> GHMSKSDYIQNMFQTKSFVDRYKYTEKLTGLYAQTLVDYSGVANTSQKPLIVLDNACGIGAVSSVLNHTLQDEAKKTWKLTCGDLSEGMLETTKRRLQDEGWVNAETKIVNALDTGLPDGHYTHVFVAFGFQSFPDANAALKECFRILASGGILASSTWQNFNWIPIMKAAIETIPGNLPFPTQKEFIALHNAGWDSESYIQSELEKLGFRDVKVIPVPKETSIPIDEFFEVCMMIIPYLLPKFWTEEQRESHEKDVPMVLRQYLQDTYGANGQVPLEAVALITTGLKP

We and others have shown that A. fumigatus effects dithiol gliotoxin S-methylation via a methyltransferase, gliotoxin thiomethyltransferase A (GtmA or TmtA) located outside the gliotoxin gene cluster. GtmA consists of two domains, a larger ‘upper’ domain containing a Rossmann-fold involved in binding the co-substrate SAM and a smaller ‘lower’ domain that changes its relative position to the upper domain in the three crystal structures described here. apo-GtmA seems to be highly flexible, as indicated by the higher B-factors. In agreement with Duell et al., who have recently published the structure of a GtmA–SAH complex in the same crystal form as described here, the cofactor binding site of GtmA is located in the upper part of a cleft between the two domains built by helix α1, sheet β2 and loop regions connecting β1–α2 and β3–β4. Our data suggest that GtmA methylates dithiol gliotoxin by a non-processive mechanism.

In order to obtain detailed insights into the enzymatic mechanism of GtmA-catalysed methyltransfer, we crystallized GtmA in the cofactor-free form and in complex with SAM and SAH, and refined the structures at 1.66 Å, 2.28 Å and 1.33 Å resolution with R-factors of Rapo = 16.8, RSAM = 19.2, RSAH = 13.9, and Rfree-values of Rfreeapo = 18.6, RfreeSAM = 23.4, RfreeSAM = 16.6, respectively. The apo form crystallized in space group P62 with one chain in the asymmetric unit, whereas the complexes appeared in two different crystal forms belonging to space group P21 with two monomers as the asymmetric unit in both cases. The flexibility is more pronounced in the lower domain, which is also evident by the finding that almost no ordered water molecules can be observed in the electron density of this region. The apo structure adopts a similar conformation as the SAH complex; however, parts of the upper domain (the first 22 residues of the N-terminus including parts of α1 and residues 86–114, including the complete secondary structure elements β3 and α4), are not visible in the electron density. In order to investigate possible structural rearrangements and gain mechanistic insights into this transformation, we structurally elucidated the GtmA-apo, GtmA–SAM and GtmA–SAH-bound structures. These structures revealed several flexible parts of the upper domain (α1, α4 and β3) which are not visible in the electron density of the apo structure. Interestingly, the two important residues Ala54 and Asp82 are part of β-strands β1 and β2, two regions connected by a disulfide bridge formed by Cys55 and Cys80 in the apo structure. This disulfide bridge appears to be reduced in the cofactor-bound structures, leading to a movement of the two β-strands towards the cofactor. We investigated the possible relevance of the disulfide bridge by carrying out microscale thermophoresis (MST) to determine the affinity of GtmA for SAM under reducing and oxidizing conditions; however, the affinity of GtmA for SAM was similar in both cases.>NFNIGSLSDQLSKQTLLISQLQVGKNRFSFKFEGRVVYKSSTFQNQQDSKYFFITAQDANNQEINMSFWQKVDQSYQTLKVGQYYYFIGGEVKQFKNNLELKFKF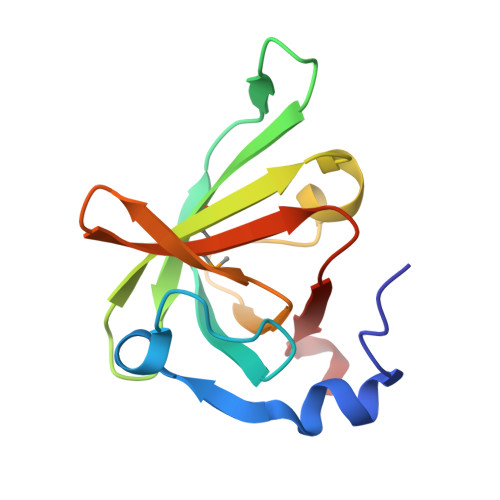GDYQIIPKETLS[2x]> MSERIVISPTSRQEGHAELVMEVDDEGIVTKGRYFSITPVRGLEKMVTGKAPETAPVMVQRICGVCPIPHTLASVEAIDDSLDIEVPKAGRLLRELTLAAHHVNSHAIHHFLIAPDFVPENLMADAINSVSEIRKNAQYVVDMVAGEGIHPSDVRIGGMAD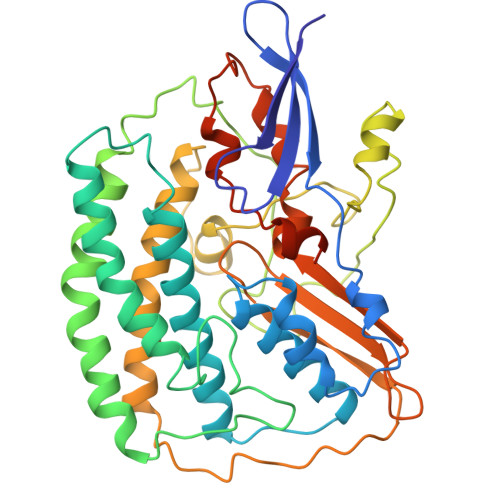NITELARKRLYARLKQLKPKVNEHVELMIGLIEDKGLPEGLGVHNQPTLASHQIYGDRTKFDLDRFTEIMPESWYDDPEIAKRACSTIPLYDGRNVEVGPRARMVEFQGFKERGVVAQHVARALEMKTALSRAIEILDELDTSAPVRADFDERGTGKLGIGAIEAPRGLDVHMAKVENGKIQFYSALVPTTWNIPTMGPATEGFHHEYGPHVIRAYDPCLSCATHVMVVDDEDKSVIKNEMVKI>[2x]SRAYDLVVIGAGSGGLEAGWNAASLHKKRVAVIDLQKHHGPPHYAALGGTCVNVGCVPKKLMVTGANYMDTIRESAGFGWELDRESVRPNWKALIAAKNKAVSGINDSYEGMFADTEGLTFHQGFGALQDNHT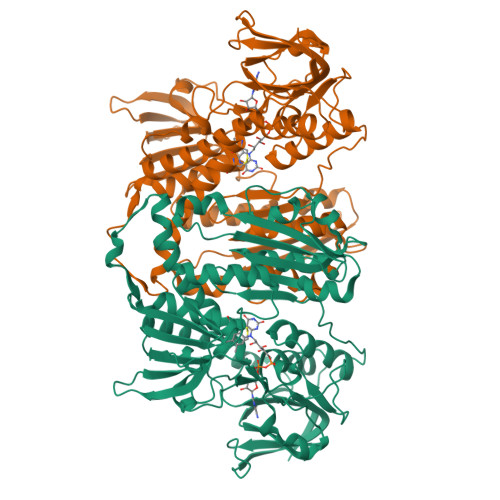VLVRESADPNSAVLETLDTEYILLATGSWPQHLGIEGDDLCITSNEAFYLDEAPKRALCVGGGYISIEFAGIFNAYKARGGQVDLAYRGDMILRGFDSELRKQLTEQLRANGINVRTHENPAKVTKNADGTRHVVFESGAEADYDVVMLAIGRVPRSQTLQLEKAGVEVAKNGAIKVDAYSKTNVDNIYAIGDVTDRVMLTPVAINEGAAFVDTVFANKPRATDHTKVACAVFSIPPMGVCGYVEEDAAKKYDQVAVYESSFTPLMHNISGSTYKKFMVRIVTNHADGEVLGVHMLGDSSPEIIQSVAICLKMGAKISDVYNTIGVHPTSAEELCSMRTPAYFYEKGKRVEKIDSNL> GPGSDNKEQTTDQPLAKDKVALLIGNMNYREHPKLKAPLVDVYELTNLLRQLDFKVVSLLDLTEYEMRNAVDEFLLLLDKGVYGLLYYAGHGYENFGNSFMVPVDAPNPYRSENCLCVQNILKLMQEKETGLNVFLLDMCRKRNDYDDTIPILDALKVTANIVFGYATCQGAEAFEIQHSGLANGIFMKFLKDRLLEDKKITVLLDEVAEDMGKCHLTKGKQALEIRSSLSEKRALTDPIQGTEYSAESLVRNLQWAKAHELPESMCLKFD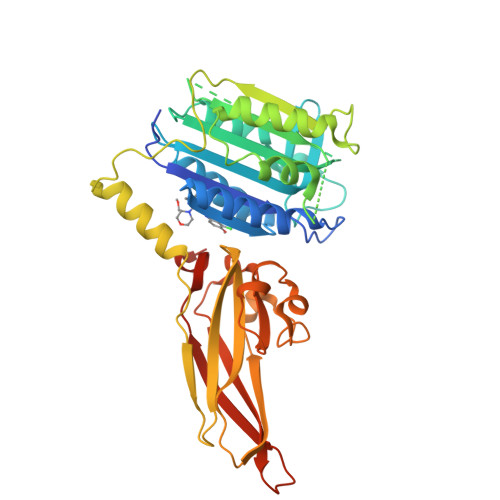CGVQIQLGFAAEFSNVMIIYTSIVYKPPEIIMCDAYVTDFPLDLDIDPKDANKGTPEETGSYLVSKDLPKHCLYTRLSSLQKLKEHLVFTVCLSYQYSGLEDTVEDKQEVNVGKPLIAKLDMHRGLGRKTCFQ>[3x]SNAMDSSASVVFMRFAPPGEE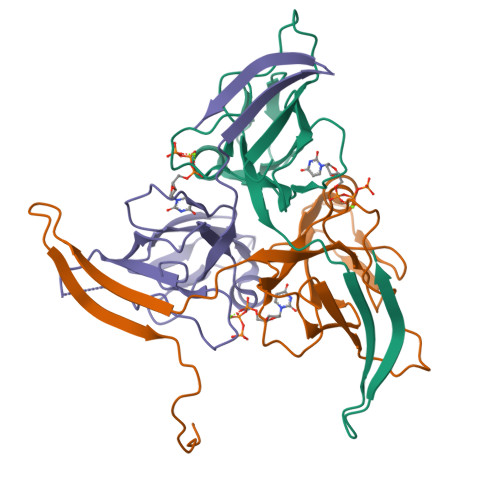TALPPRRATPGSVAYDLFPSEEMDIEPMGLAKISTGYGIDKFPDGCYGQIVSRSGMTWKNNTSVPTGTINVDYRGELKVILRNHSAEKSVPIRKGTSIAQLIFLRYCDVEEEQIVYINETTGERTIIDSSSKKDNKNQAESVRGTGGFGSTDN>[2x]MPYVEIIEQPKQRGMRFRYKCEGRSAGSIPGERSTDTTKTHPTIKINGYTGPGTVRISLVTKDPPHRPHPHELVGKDCRDGYYEADLCPDRSIHSFQNLGIQCVKKRDLEQAISQRIQTNNNPFHVPIEEQRGDYDLNAVRLCFQVTVRDPAGRPLLLTPVLSHPIFDNRAPNTAELKICRVNRNSGSCLGGDEIFLLCDKVQKEDIEVYFTGPGWEARGSFSQADVHRQVAIVFRTPPYADPSLQAPVRVSMQLRRPSDRELSEPMEFQYLPDTDDRHRIEEKRKR

Among the NF-κB family of dimeric TFs, the p50:RelA heterodimer and the RelA:RelA homodimer are most ubiquitous and well-studied. These dimers bind with high affinity to ∼10-bp sequences (κB sites), with a general consensus of GGGRNNYYCC, defined over 35 years ago. Several studies indicate binding of various NF-κB dimers to thousands of degenerate κB sites with a wide gradient in affinity. Within the promoters and enhancers of NF-κB-responsive genes, we identified clusters of non-consensus κB DNA sites, many exhibiting low affinity for NF-κB in vitro.

Sequence-specific binding at the weak κB site (2ΔS) was retained upon mutation of strong site for both dimers, demonstrating that NF-κB has the capacity to bind this weak motif. To further evaluate whether the binding by NF-κB dimers to weak κB sites is specific and authentic, we determined the crystal structure of RelA homodimer in complex with a weak κB site (−5G−4G−3G−2  C−1  T0T+1T+2T+3C+4C) present in the promoter of the Cxcl2 gene (the non-cognate base pairs are underlined and the pseudo-dyad axis separating the two halves of the κB site is marked 0T). The Arg33 and Arg35 engaged to the −4G−3G of one half-site, as predicted. However, the presence of non-cognate bases (−2C−1T compared to −2A−1A, the cognate bases for the RelA homodimer) influenced the global DNA architecture such that Arg187 is positioned slightly differently, but more importantly, R41 could not engage with −5G of this weak site. This altered protein–DNA contact likely entails the weaker interaction, which nonetheless is specific. Taken together, these results reflect an enrichment of weak κB motifs in the regulatory regions of NF-κB target genes, which can indeed be recognized specifically by RelA; however, a more elaborate mechanism must underlie an efficient occupancy of these weaker sites. Interestingly, X-ray structural studies revealed that the global nature of protein–DNA interaction is preserved regardless of the difference in binding affinity and despite both the protein and DNA undergoing conformational adjustments in forming the complex. The in vitro affinity of individual weak κB sites to NF-κB RelA homodimer or p50:RelA heterodimer is often undetectable (i.e. Kd > ∼1500 nM). These sites often deviated from the consensus at several bases.> SCPDACCPHGSSGLRCTRDGALDSLHHLPGAENLTELYIENQQHLQHLELRDLRGLGELRNLTIVKSGLRFVAPDAFHFTPRLSRLNLSFNALESLSWKTVQGLSLQELVLSGNPLHCSCALRWLQRWEEEGLGGVPEQKLQCHGQGPLAHMPNASCGVPTLKVQVPNASVDVGDD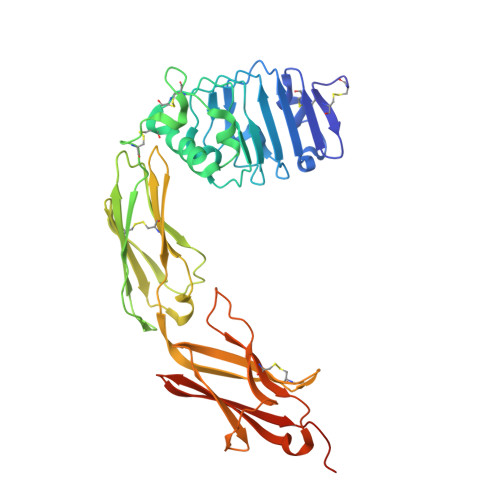VLLRCQVEGRGLEQAGWILTELEQSATVMKSGGLPSLGLTLANVTSDLNRKNLTCWAENDVGRAEVSVQVNVSFPASVQLHTAVEMHHWCIPFSVDGQPAPSLRWLFNGSVLNETSFIFTEFLEPAANETVRHGCLRLNQPTHVNNGNYTLLAANPFGQASASIMAAFMDNPAAAHHHHHHHH>NSINDSKILSLQNKKNALVDTSGYNAEVRVGDNVQLNTIYTNDFKLSSSGDKIIVNLNNNILYSAIYENSSVSFWIKISKDLTNSHNEYTIINSIEQNSGWKLCIRNGNIEWILQDVNRKYKSLIFDYSESLSHTGYTNKWFFVTITNNIMGYMKLYINGELKQSQKIEDLDEVKLDKTIVFGIDENIDENQMLWIRDFNIFSKELSNEDINIVYEGQILRNVIKDYWGNPLKFDTEYYIINDNYIDRYIAPESNVLVLVQYPDRSKLYTGNPITIKSVSDKNPYSRILNGDNIILHMLYNSRKYMIIRDTDTIYATQGGECSQNCVYALKLQS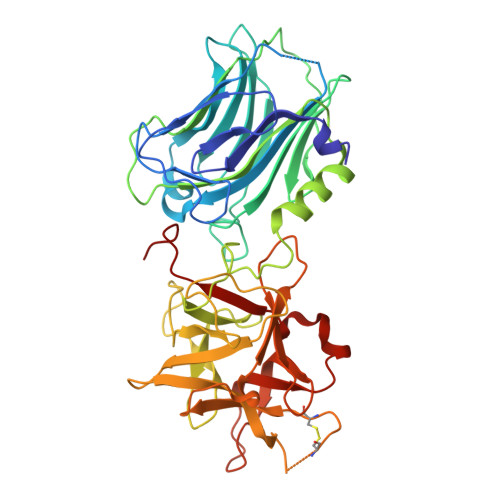NLGNYGIGIFSIKNIVSKNKYCSQIFSSFRENTMLLADIYKPWRASFKNAYTPVAVTNYETKLLSTSSFWKFISRDPGWVE[4x]> MAYLTEKIDLYGDNGKVLESDIPLEAVTPVQNPAVRELASIFKRSVAVNLGGAQKALSTGHYANEYIHFPDIPNKDKLGIKSSPGGKYPPKSVKVRTMDLPLVDDADDIAARLKERLQVNPDDGTEVRVMKKGNVLYVKISEQLANTGVEYTTALTTTAQAMTDLVMEKYDLDFHASPLVHCAFYGRYPQTYEFMGGNVISLLAASCANEGPGFAMRNIMANHIVAATRKRTLEAVALSSTLEAIGHVEMGDAIGRWRRWQALVHACQGLNANNVVYDLVKEAGHGCTGDVVAATVGRALEDGIISVKKTLPSGYKFYTANDPSMWNAYVCAGLVAAVIVNQGAARAAQGVSSTLLYFNDLIEHETGLPHAGYGDGMGNGVSFSFFSHAIYGGGSPGIFSGNHIVTRHSKGFAIPVIAAA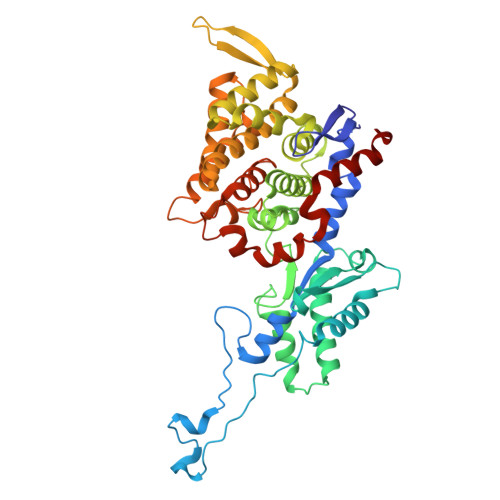VSLDSGTAVYGPEATSGLVGDIFGEVDLIRRPMEAIASAAAEIKDKF> ADV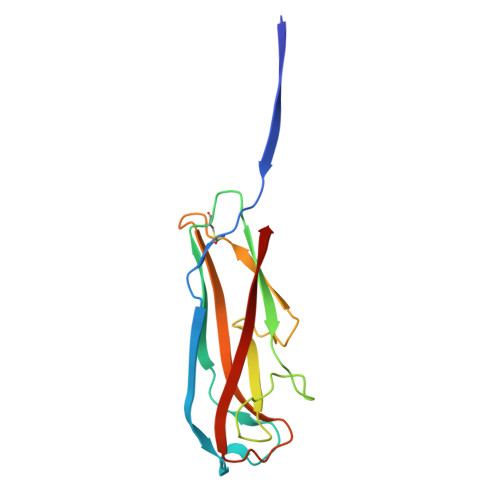TITVNGKVVAKPCTVSTTNATVDLGDLYSFSLMSAGAASAWHDVALELTNCPVGTSRVTASFSGAADSTGYYKNQGTAQNIQLELQDDSGNTLNTGATKTVQVDDSSQSAHFPLQVRALTVNGGATQGTIQAVISITYTYS>[3x]GPLGSPEFGYWITCCPTCDVDINTWVPFYSTELN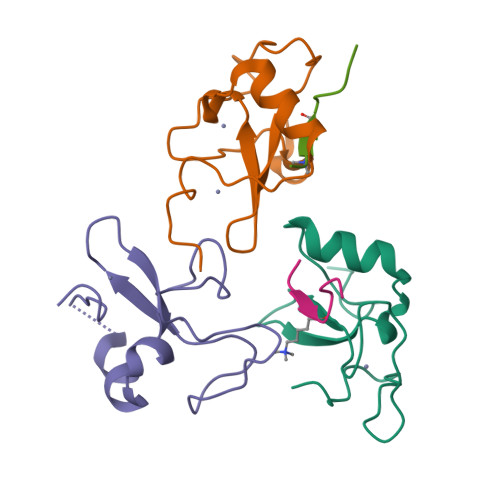KPAMIYCSHGDGHWVHAQCMDLEERTLIHLSEGSNKYYCNEHVQIARA;>[2x]ARTKQTARK> QPHIIQLKNETTYENGQVTLVCDAEGEPIPEITWKRAVDGFTFTEGDKSLDGRIEVKGQHGSSSLH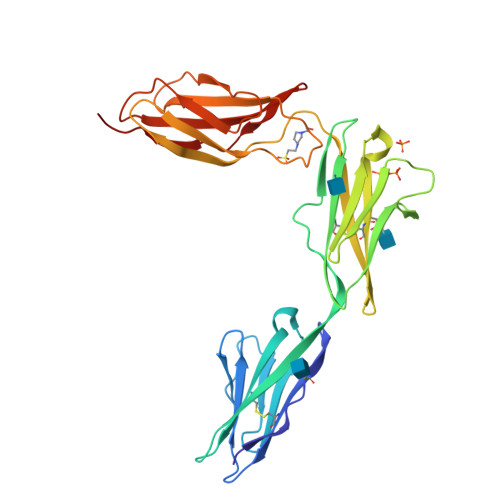IKDVKLSDSGRYDCEAASRIGGHQKSMYLDIEYAPKFISNQTIYYSWEGNPINISCDVKSNPPASIHWRRDKLVLPAKNTTNLKTYSTGRKMILEIAPTSDNDFGRYNCTATNHIGTRFQEYILALADVPSSPYGVKIIELSQTTAKVSFNKPDSHGGVPIHHYQVDVKEVASEIWKIVRSHGVQTMVVLNNLEPNTTYEIRVAAVNGKGQGDYSKIEIFQTLPV> KRKRKR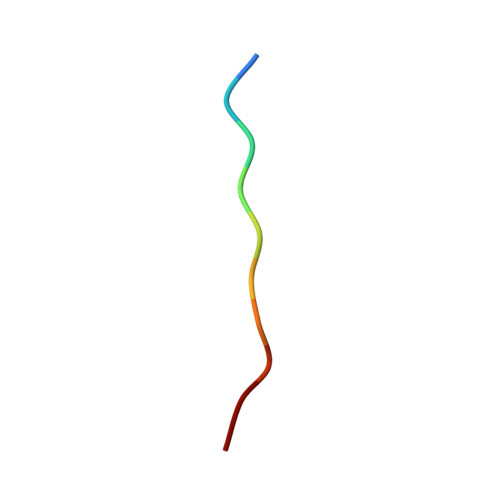KRKR>SNAMSKKAELAELVKELAVVHGKVTLSSGKEADYYVDLRRATLHARASRLIGELLRELTADWDYVAVGGLTLGADPVATSVMHADGREIHAFVVRKEAKKHGMQRRIEGPDVVGKKVLVVEDTTTTGNSPLTAVKALREAGAEVVGVATVVDRATGAADVIAAEGLEYRYILGL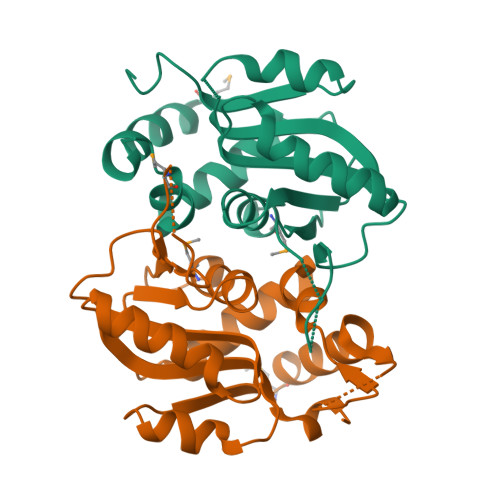EDLGLA[2x]>GAMGSRLYDRRSIFDAVAQSNCQELESLLPFLQRSKKRLTDSEFKDPETGKTCLLKAMLNLHNGQNDTIALLLDVARKTDSLKQFVNASYTDSYYKGQTALHIAIERRNMTLVTLLVENGADVQAAANGDFFKKTKGRPGFYFGELPLSLAACTNQLAIVKFLLQNSWQPADISARDSVGNTVLHALVEVADNTVDNTKFVTSMYNEILILGAKLHPTLKLEEITNRKGLTPLALAASSGKIGVLAYILQREIHEPECRHLSRKFTEWAYGPVHSSLYDLSCIDTCEKNSVLEVIAYSSSETPNRHDMLLVEPLNRLLQDKWDRFVKRIFYFNFFVYCLYMIIFTAAAYYRPVEGLPPYKLKNTVGDYFRVTGEILSVSGGVYFFFRGIQYFLQRRPSLKSLFVDSYSEILFFVQSLFMLVSVVLYFSQRKEYVASMVFSLAMGWTNMLYYTRGFQQMGIYAVMIEKMILRDLCRFMFVYLVFLFGFSTAVVTLIEDGKYNSLYSTCLELFKFTIGMGDLEFTENYDFKAVFIILLLAYVILTYILLLNMLIALMGETVNKIAQESKNIWKLQRAITILDTEKSFLKCMRKAFRSGKLLQVGFTPDGKDDYRWCFRVDEVNWTTWNT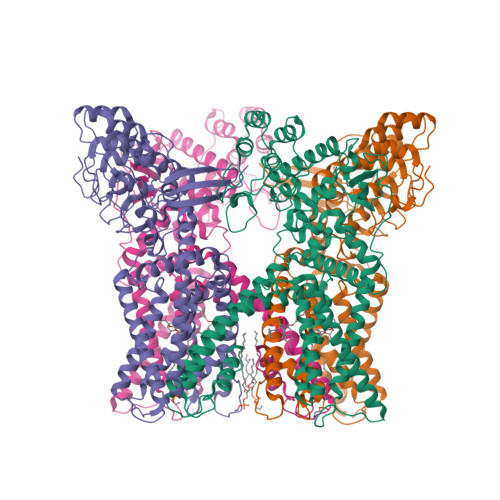NVGIINEDPG[4x]> MSMLAKIAKNVVKTQALKNTTAAQTPSFQAPGNQDKILKWISTLSNKATTGESRSYCTQLSSLVSFYNKQHVEQIPTIDFNEWKSVISTQGLVDKVKENYESLIKEQYN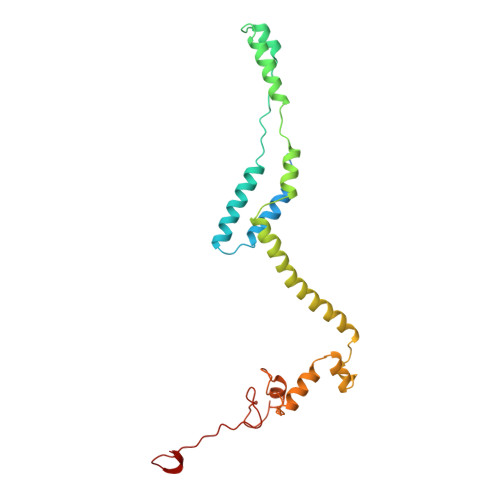TDAISKQISSASSKALDDIENELSFHAAIWLNAYADYTMFLFELEEYNDPNDYLMHENFDFFRGLETELEELTETHNYIPGAKDDVNLRGYLATQFAWGKKVISFYRHPADDFKCAKATKNMLGR> MPEQPFIVLGQEEYGEHHSSIMHCRVDCSGRRVASLDVDGVIKVWSFNPIMQTKASSISKSPLLSLEWATKRDRLLLLGSGVGTVRLYDTEAKKNLCEININDNMPRILSLACSPNGASFVCSAAAPSLTSQVDFSAPDIGSKGMNQVPGRLLLWDTKTMKQQLQFSLDPEPIAINCTAFNHNGNLLVTGAADGVIR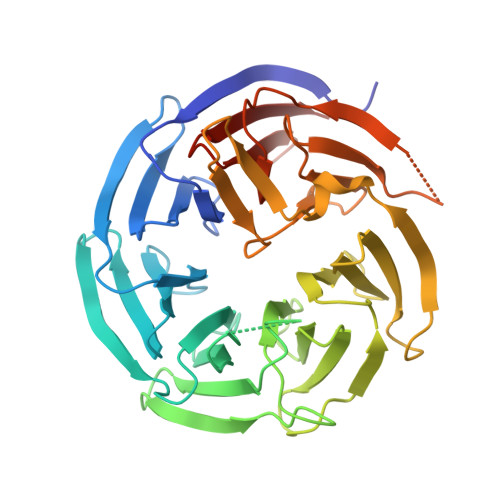LFDMQQHECAMSWRAHYGEVYSVEFSYDENTVYSIGEDGKFIQWNIHKSGLKVSEYSLPSDATGPFVLSGYSGYKQVQVPRGRLFAFDSEGNYMLTCSATGGVIYKLGGDEKVLESCLSLGGHRAPVVTVDWSTAMDCGTCLTASMDGKIKLTTLLAHKAHHHHHH2-{5-[AMINO(IMINIO)METHYL]-1H-BENZIMIDAZOL-2-YL}-6-ISOBUTOXYBENZENOLATE | C18 H20 N4 O2 | 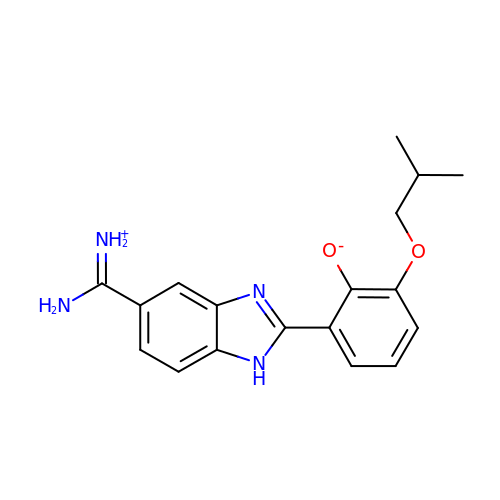HSHVHNIOQTZSOQ-UHFFFAOYSA-N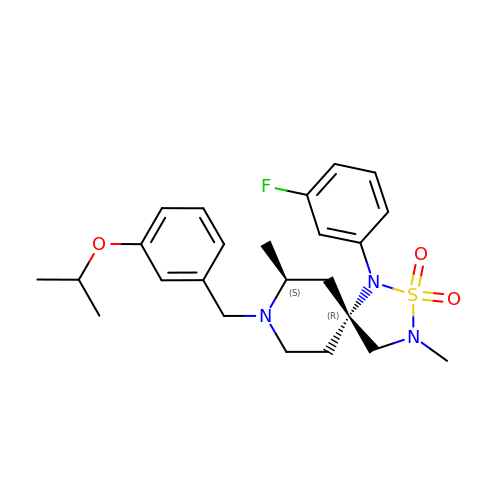(5R,7S)-1-(3-fluorophenyl)-3,7-dimethyl-8-[3-(propan-2-yloxy)benzyl]-2-thia-1,3,8-triazaspiro[4.5]decane 2,2-dioxide | C24 H32 F N3 O3 S | CVPXZTQJPHYLAQ-YADARESESA-N>[4x]GKAFDDGAFTGIREINLSYNKETAIGDFQVVYDLNGSPYVGQNHKSFITGFTPVKISLDFPSEYIMEVSGYTGNVSGYVVVRSLTFKTNKKTYGPYGVTSGTPFNLPI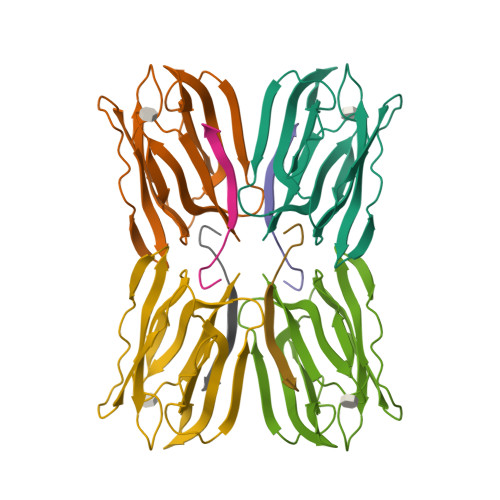ENGLIVGFKGSIGYWLDYFSMYLSL;>[4x]NEQSGKSQTVIVGSWGAKVS Several Vibrio species use ToxR to mediate bile resistance, and a few pathogenic species have co-opted ToxR for virulence induction. While over-expression of ToxR can lead to ToxR regulon transcription, under physiological conditions ToxR requires ToxS, an integral membrane protein with a periplasmic domain, for full activity. In wild type ToxR, these cysteines are known to form either an intra-chain disulfide bond or a disulfide linked homodimer, which is present when toxS is deleted in V. cholerae. The disulfide bonded ToxR periplasmic domain consists of 5 β-strands and 2 α-helices forming an α/β fold.

The dbToxRp from V. vulnificus, which shares 55.2% identity to the V. cholerae ToxR periplasmic domain, readily crystallized. The crystal structure of V. vulnificus intra-chain disulfide ToxR periplasmic domain (Vv-dbToxRp) was solved by molecular replacement using a selenomethionine (SeMet) labeled structure to 1.25 Å (Statistics are shown in Table S1). Given the two structures are essentially the same we focused on analyzing the native structure. The 5 β-strands are arranged in a β-sheet with one side packed against the two α-helices, through hydrophobic interactions. Interactions of note include a Pi-Pi stacking interaction between the Tyr236 from α1 and Tyr263 from β4 in the hydrophobic core of the protein. A sulfate ion was found in the structure, stabilized by the side chain of Arg203 and the amide nitrogens of Leu222 and Gln223. Finally, the disulfide bond between Cys232 and Cys289 covalently attaches α2 to α1 stabilizing the structure. Interestingly, the density of the α2-β5 loop (residues 281–284) was poorly defined. In addition, the α2-β5 loop has the highest B-factors in the structure (Fig. 3d last panel). Taken together this indicates the loop is flexible. Therefore, we hypothesize a major role of the disulfide bond is to stabilize the structure, and importantly the ToxS binding region, by constraining this flexible loop as well as the relatively short helix, α2, which follows it. Interestingly, MatchMaker35 aligned the VtrA periplasmic domain to dbToxRp with the lowest all atom RMSD of 5.5 Å, suggesting despite the placement of VtrA in the DALI search the VtrA and ToxR periplasmic domains are structural homologs.

> MAHHHHHHTNPSESKFRLLENVNGVEVLTPLNHPPLQAWMPSIRQCVNKYAETHTGDSAPVKVIATGGQGNQLILNYIHTLPHSNENVTLRIFSEQNDLGSICK Methionine adenosyltranferases (S-adenosylmethionine synthase, MetK, EC 2.5.1.6, MAT) catalyse the synthesis of S-adenosylmethionine (SAM) from adenosine triphosphate (ATP) and methionine. MAT is abundant in all three domains of life, and the cofactor SAM is essential for a variety of different enzymatic reactions. We describe the initial characterisation and the crystal structure of the methionine adenosyltransferase from the hyperthermophilic archaeon Thermococcus kodakarensis. As described for other archaeal methionine adenosyltransferases the enzyme is a dimer in solution and shows high temperature stability.

The crystals belonged to the monoclinic space group C2, with four monomers of the enzyme per asymmetric unit. TkMAT appears as a dimer in solution, but was found in the crystal packing as a tetramer, which is quite similar to those reported for the MATs from E. coli or R. norvegicus. The four monomers of TkMAT within the asymmetric unit are similar in structure, but while the monomers within each homodimer aligned with a root-mean-squared displacement (r.m.s.d.) for all atoms of 0.63 Å (chains A, B) and 0.64 Å (chains C, D), the corresponding monomers in different dimers were nearly identical (r.m.s.d. of 0.14 Å and 0.15 Å). These differences in structure manifest primarily in the β-sheet and the adjacent loops of the C-terminal domain, where a significant asymmetry of the functional dimer of up to 4 Å is present, a similar behaviour can also be observed in other MAT structures. Compared to bacterial and eukaryotic MATs, TkMAT and MjMAT contain an additional β-strand at the N-terminus (amino acids 1-17 in TkMAT) that forms a part of the C-terminal domain. In archaeal MATs the additional β-strand extends the β-sheet of the C-terminal domain to match the four-stranded sheets found in the N-terminal and central domains, and therefore might add to the higher stability of archaeal MATs by providing a direct connection between the N- and C-termini of the peptide chain within a stable secondary structure. A major difference between TkMAT and other MAT structures without any bound ligands is that the helix covering the active site is completely defined in the structure. Until now the flexible loop was thought to be disordered in the open conformation, however all four monomers in the asymmetric unit of the TkMAT crystal showed the same ordered helix in the open structure. The higher intrinsic stability of the thermophilic enzyme could explain why this region is well defined in the structure of TkMAT. The most obvious examples for such different stabilising strategies are the hydrogen-bonding networks coordinating the carboxyl group of the methionine moiety, and the adenine amino group.

>[4x]MAGKVRNIVVEELVRTPVEMQKVELVERKGIGHPDSIADGIAEAVSRALSREYVKRYGIILHHNTDQVEVVGGRAYPQFGGGEVIKPIYILLSGRAVEMVDREFFPVHEIALKAAKDYLRKAVRHLDLEHHVIIDSRIGQGSVDLVGVFNKAKKNPIPLANDTSFGVGYAPLSETEKIVLETEKYLNSDEFKKKYPAVGEDIKVMGLRKGDEIDLTIAAAIVDSEVDNPDDYMAVKEAIYEAAKGIVESHTERPTNIYVNTADDPKEGIYYITVTGTSAEAGDDGSVGRGNRVNGLITPNRHMSMEAAAGKNPVSHVGKIYNILSMLIANDIAEQVEGVEEVYVRILSQIGKPIDEPLVASVQIIPKKGYSIDVLQKPAYEIADEWLANITKIQKMILEDKVNVF>SNAMSTSL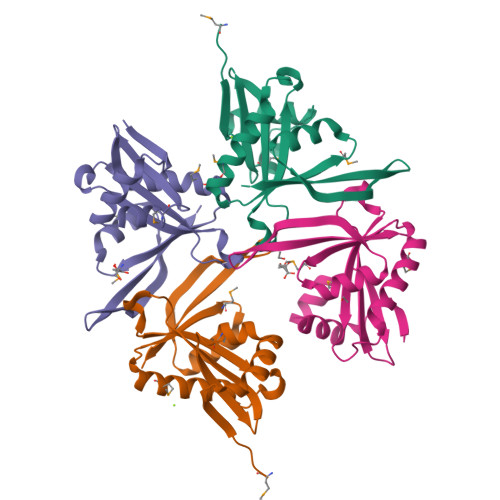TIRLVAEADWPALHALDQIIWTKKNTPAEIQPLSLAAYQEKMKDETIFVAISGQQLAGFIEVHPPTSLAAHQKQWLLSIGVSPDFQDQGIGGSLLSYIKDMAEISGIHKLSLRVMATNQEAIRFYEKHGFVQEAHFKEEFYINGHYCDDYQYAYFIEK[4x]> MGSDSIDTPNYDVQKHINKLCGMLLITED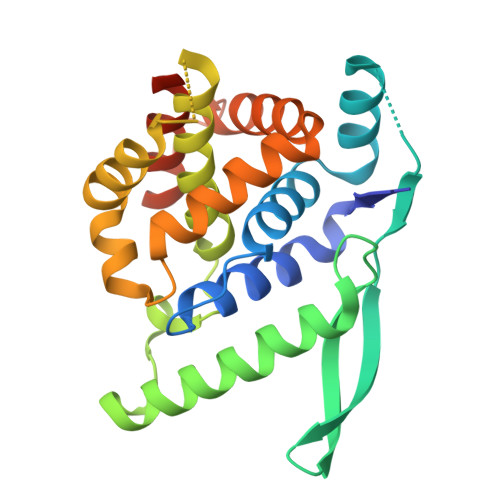ANHKFTGLIGMLYAMSRLGREDTIKILRDAGYHVKANGVDVTTHRQDINGKEMKFEVLTLASLTTEIQINIEIESRKSYKKMLKEMGEVAPEYRHDSPDCGMIILCILALVITKLAAGDRSGLTAVIRRANNVLKNEMKRYKGLLPKDIANSFYEVFEKHPHFIDVFVHFGIAQSSTRGGSRVEGIFAGLFMNAYGLEHHHHHH>[4x]MGATRIQAVYRDTGVEAYRDNPFIEALPPLQESVNSAASLKSSLQLTSSDLQKSRVIRAHTICRIPDDYFQPLGTHLLLSERISVMIRGGYVGRNPKTGDLQKHLQNGYERVQTGELETFRFEEARSTAQSLLLIGCSGSGKTTSLHRILATYPQVIYHRELNVEQVVYLKIDCSHNGSLKEICLNFFRALDRALGSNYERRYGLKRHGIETMLALMSQIANAHVLGLLVIDEIQHLSRSRSGGSQEMLNFFVTMVNIIGVPVMLIGTPKAREIFEADLRSARRGAGFGAIFWDPIQQTQRGKPNQEWIAFTDNLWQLQLLQRKDALLSDEVRDVWYELSQGVMDIVVKLFVLAQLRALALGNERITAGLLRQVYQDELK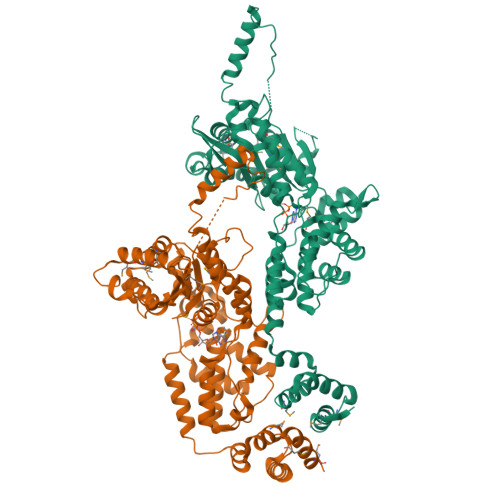PVHPMLEALRSGIPERIARYSDLVVPEIDKRLIQLQLDIAAIQEQTPEEKALQELDTEDQRHLYLMLKEDYDSSLLIPTIKKAFSQNPTMTRQKLLPLVLQWLMEGETVVSELEKPSKSKKVSPNSSSVDKLAAALEHHHHHH>HLKPEMIEKLNEQMNLELYSSLLYQQMSAWCSYHTFEGAAAFLRRHAQEEMTHMQRLFDYLTDTGNLPRINTVESPFAEYSSLDELFQETYKLEQLITQKINELAHAAMTNQDYPTFNFLQWYVSEQHEEEKLFKSIIDKLSLAGKSGEGLYFIDKEL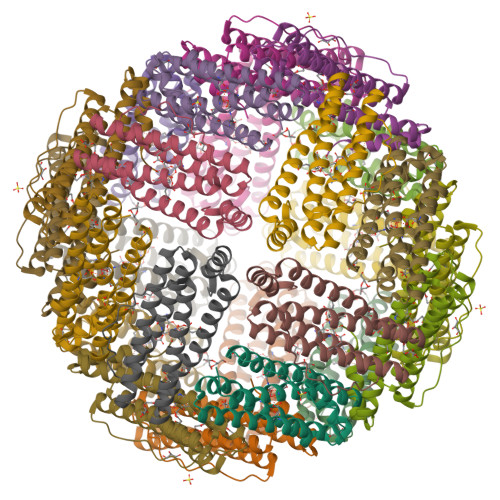STLDTQN[6x]>[2x]SNAMSQFMNLEGKVALVTGASRGIGKAIAELLAERGAKVIGT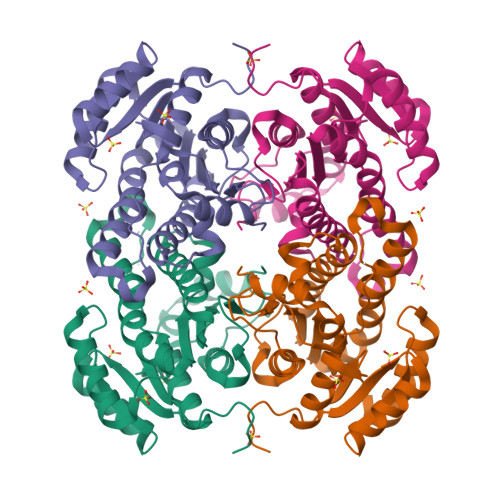ATSESGAQAISDYLGDNGKGMALNVTNPESIEAVLKAITDEFGGVDILVNNADITRDNLLMRMKEEEWSDIMETNLTSIFRLSKAVLRGMMKKRQGRIINVGSVVGTMGNAGQANYAAAKAGVIGFTKSMAREVASRGVTVNTVAPGFIETDMTKALNDEQRTATLAQVPAGRLGDPREIASAVAFLASPEAAYITGETLHVNGGMYMI>MAKCSKGRTASNDACCVWFDVLDDIQENLFDGGECGEEVHESLRLTFHDAIGFSPALTRQGKFGGGGADGSIMLFSDIETNFAANNGVDDIVEQQKPIAIKHQVSFGDFIQFAGAVGSSNCAGGPRIQFLAGRSNVTKPSPDHLVPEPFDSVTSILARMGDAGFKPDEVVALLASHSVAAQDTIDPKLAGHPFDSTPSDFDSQFFVETLLKGTLIPGDSLHKGQVKSPLPGEFRLQSDELLARDSRTSCEWQSFISNPNSMVPKFERAMAKMATLGQNPKKLIDCSEVIPVPRGRVKQPTLPAGKTIKDIEASCRKAPFPRLPTDKGTFTSILPVPSS[2x]

The heterologous expression of the POD genes from the P. ostreatus genome, and subsequent kinetic studies, reveal a peroxidase array consisting of three VPs and six MnPs. The VP1 and MnP4 crystal structures were solved as representative for the two POD families present in the P. ostreatus genome. The overall structure of VP1 and MnP4 showed a heme group dividing the protein into a distal largely helical domain (formed by four main helices and two to three small ones) with one structural calcium ion, and a proximal domain composed by another six helices and a non-ordered region stabilized by a second calcium ion. The site where this takes place is conserved and comprises three acidic residues (E36/E40/D175 in VP1 and E36/E40/D181 in MnP4) located near the heme propionate occupying the most internal position with respect to the main access channel.

The resulting inventory revealed the absence of lignin peroxidases (LiPs) and the presence of three versatile peroxidases (VPs) and six manganese peroxidases (MnPs), the crystal structures of two of them (VP1 and MnP4) were solved at 1.0 to 1.1 Å showing significant structural differences. Concerning short MnP, whose crystal structure is now solved for the first time (from P. ostreatus MnP4), its main structural difference from P. chrysosporium long MnP concerns the existence of a more exposed Mn oxidation site, due to the absence of the C-terminal extension that in P. chrysosporium MnP (with a total of 357 residues) is partially fixed by a fifth disulfide bridge. The oxidation of lignin-related substrates was not detected in MnP4, where the active tryptophan is substituted by an alanine (left). At this site, the P56 to G59 loop of VP1 presents a six-residue insertion in MnP4 forming a small extra helix that protrudes into the solvent. Also, residues A130 and V131 in this VP1 region adopted a different conformation with respect to V135 and T136 in MnP4. These changes allow the F62 hydrophobic side chain of MnP4 to interact with K137 and, due to this interaction, the hydroxyl group of T136 interacts with one of the waters coordinating the distal calcium ion. Most of them involve the change of small hydrophobic side chains in VP1 for large hydrophilic side chains, such as the substitution of G290 in VP1 by K296 in MnP4. This lysine has interactions with D198 and D200, which are directly involved in the coordination of the proximal calcium. When the MnP4 crystal structure was solved, a striking observation was the high number of solvent-exposed lysines (a total of 20) and other basic residues (up to a total of 34). Another noteworthy characteristic of MnP4 is the high number of surface-exposed lysines (up to a total of 20) and other alkaline residues (up to a total of 35) compared with the other P. ostreatus PODs, which would result in a higher net positive charge of the protein and increased stability at acidic pH.>STFVAKDGTQIYFKDW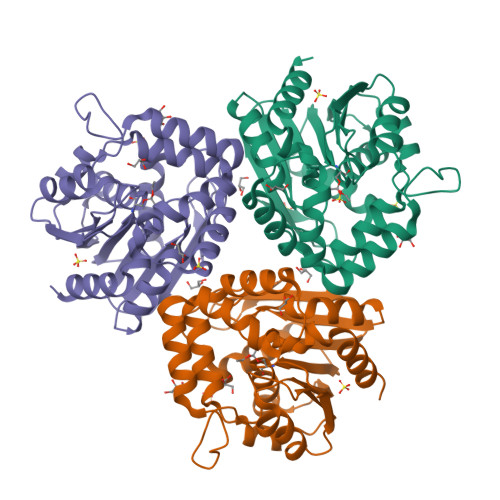GSGKPVLFSHGWPLDADMWEYQMEYLSSRGYRTIAFDRRGFGRSDQPWTGNDYDTFADDIAQLIEHLDLKEVTLVGFSMGGGDVARYIARHGSARVAGLVLLGAVTPIFGQKPDYPQGVPLDVFARFKTELLKDRAQFISDFNAPFYGINKGQVVSQGVQTQTLQIALLASLKATVDCVTAFAETDFRPDMAKIDVPTLVIHGDGDQIVPFETTGKVAAELIKGAELKVYKDAPHGFAVTHAQQLNEDLLAFLKR[6x]>FTLIELMIVIAIVGILAAVALPAYQDYTARAQVSEAILLAEGQKSAVTEYYLNHGKWPENNTSAGVASSPTDIKGKYVKEVEVKNGVVTATMLSSGVNNEIKG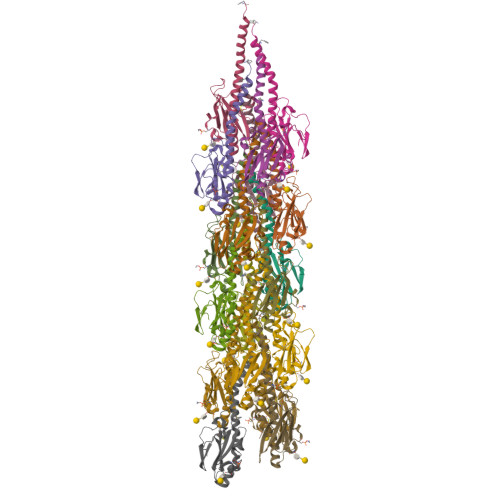KKLSLWARRENGSVKWFCGQPVTRTDDDTVADAKDGKEIDTKHLPSTCRDNFDAK[18x]> SKPRNQQQVCPLQNVPAWGYSLYKGIDMSVPLAYDPNNELGDLKDVFPSAV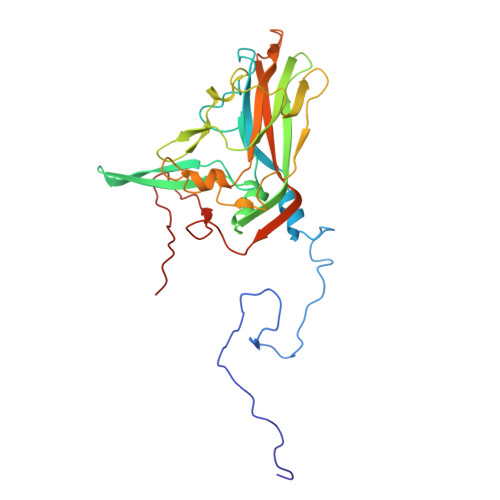DEMAIGYVCGNPAVKHVLTWKTTDAIQKPIANGDDWGGVIPVGMPCYSKSIRTIKISETENRETEVIDAAPCEYVANMFSYWRATMCYRITVVKTAFHTGRLEIFFEPGVIPVKPTVNNIGPDQDQLTGAVAPSDNNYKYILDLTNDTEVTIRVPFVSNKMFLKTAGIYGANSENNWNFHESFSGFLCIRPVTKLMAPDTVSDNVSIVVWKWAEDVVVVEPKPLTSGPTQVYRPPPTASAAVEVLNVELQ> MAQDALSDGFVRLCIDPSLNFFGEGCKILVEGQMTDDGSATPDAVTCVTSELDIIERFGQGSVLTESLRKVFCTCKSGVSVYALPREDAAAGVKAVYTLTIAGPATTDGRVQLYM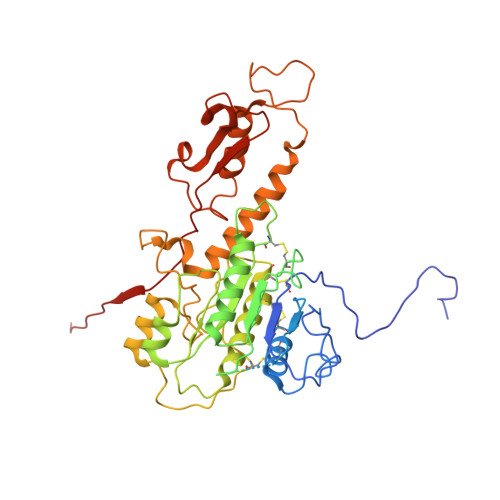GEAEYAVDIGVDAGDTATDIAAAIVAAISPDFPYAATAAAGVITLTARNAGTIGNHLSVIYTNLGSCTSVTPEGVTVTFAQTTAGSVNPTPNDYATVVNECCFAVYVLSSDDTDWQENLRDWIRSAWDCSKPQCFGHGYVFNKGTLGQVLADGDNSAELSRLALPTTYPVLPYLTNAAYGALSACSTCNNPELNIQGQTFGLLSCINMPESCTPGWTFGEVTQLQANGFVVSGPSTTSGQGNYTSPYIYNDVTNYLRDEKNRPNATFRDASSRRLAAATGVALAEFLQQFNGLAVFTKNTNIRTGIIGTNPRLMLGKIRKWAQDNVGTLFSEFDNINEDIQLLTDFEVQPKCVGQPGIFHLNMRYRPPVRGARINVNMAPALFDNCDR> MEYSNPVIKGFYPDPSICRVGSDYYLVTSSFQYFPGVPIFHSTNLINWNKIGYCLIRPSQLMLNNATNRSGIFAPTLRYHEGIFYLITTNVTLKKNFIVMSEDLQGEWSEPIWIDGWGGIDPSLFFDNDGKVYITGTNDNARGEELGIYQAEIDLKKGSIIGERKLIWKGTGGSYPEAPHLYKVNGWYYLLIAEGGTEYGHMVTVARSKYPFGPFESCPFNPILTHRSTNHPLQAIGHADIVQYHDGSWWAVFHGTRPISYPPKHHLGR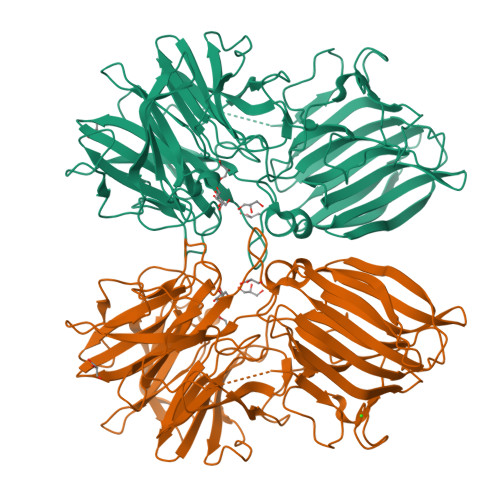ETCLAPIKWTDDGWPIIGYNGRIDIKMDAGYLPVKEKNIGDEIIEDDFNSDIFSTDWNFIQNPRLEHYSLKGRPSWLKMRGTEKTLNDINSPTFIGRRQEHFVCNVSTLLEFKPNQDNEEAGLTVYMNEKHHYEIALTKKNGRINVVLKKTVGDIQVVVNSLEYFSNTIIFSIQANPEEYKFSFVDPNTGQTYLLGTGLTTLLSTEVAGGFTGVYFGLYATGNGKVCTAPAFFDWFKYIPEIKGELNSKLEGKPIPNPLLGLDSTRTGHHHHHH> CACGAGCCTGATCGGACAAGATCCGCTAGCGAGTTAGCCTAG;> GAGCAGCCTGTACGGACATCAGTCTCTGCTAGATCGTCAGCA;> AACCTACCTGGCAGGACGACT;> TGCTAGGCTAACTCGCTAGCGGATCTTGTGGCTGC;> TTAGTCGTGGCTCG;> TCTGCTGACGATCTAGC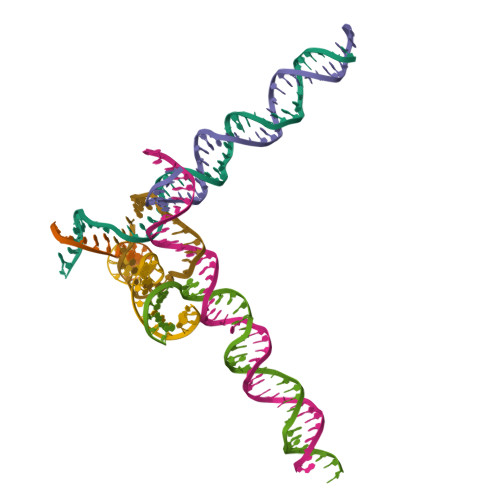AGAGACTGATGTGGTAGG;> TCACCTGCCACCGTACACCGA>[2x]SERPSPPVNLTSSDQTQSSVQLKWEPPL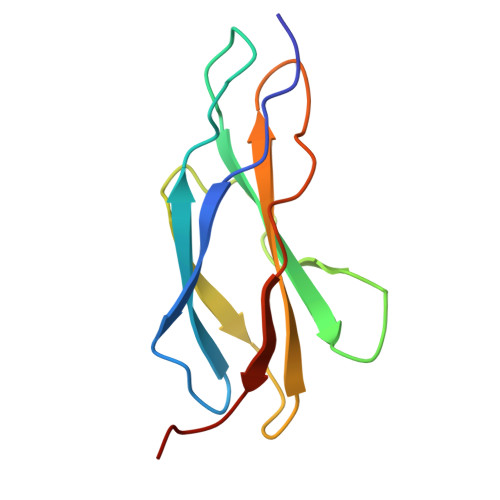KDGGSPILGYIIERCEEGKDNWIRCNMKLVPELTYKVTGLEKGNKYLYRVSAENKAGVSDPSEILGPLTADDAFVE4-(4-methylpiperidin-1-yl)-6-[4-(trifluoromethyl)phenyl]pyrimidin-2-amine | C17 H19 F3 N4 | 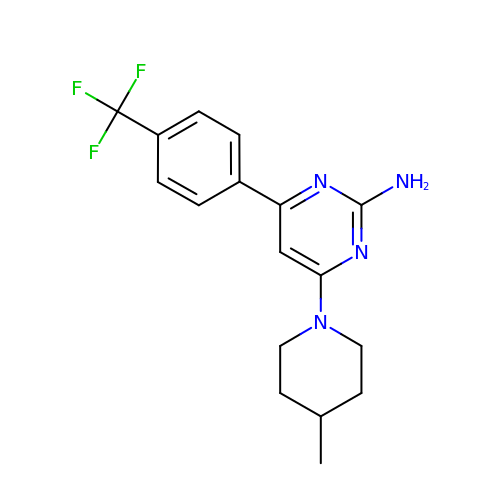YZEUYKXNCFTYAI-UHFFFAOYSA-N>[4x]GAMGSRLYDRRSIFDAVAQSNCQELESLLPFLQRSKKRLTDSEFKDPETGKTCLLKAMLNLHNGQNDTIALLLDVARKTDSLKQFVNASYTDSYYKGQTALHIAIERRNMTLVTLLVENGADVQAAANGDFFKKTKGRPGFYFGELPLSLAACTNQLAIVKFLLQNSWQPADISARDSVGNTVLHALVEVADNTVDNTKFVTSMYNEIL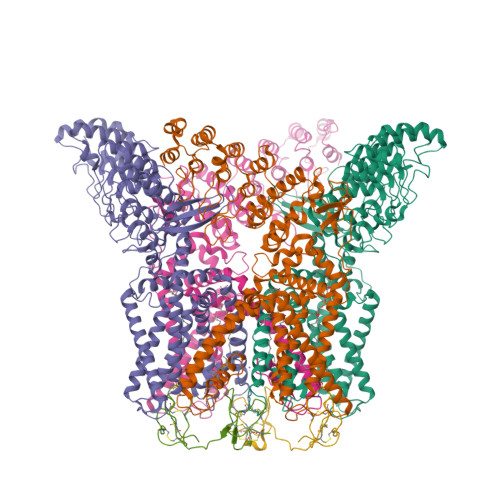ILGAKLHPTLKLEEITNRKGLTPLALAASSGKIGVLAYILQREIHEPECRHLSRKFTEWAYGPVHSSLYDLSCIDTCEKNSVLEVIAYSSSETPNRHDMLLVEPLNRLLQDKWDRFVKRIFYFNFFVYCLYMIIFTAAAYYRPVEGLPPYKLKNTVGDYFRVTGEILSVSGGVYFFFRGIQYFLQRRPSLKSLFVDSYSEILFFVQSLFMLVSVVLYFSQRKEYVASMVFSLAMGWTNMLYYTRGFQQMGIYAVMIEKMILRDLCRFMFVYLVFLFGFSTAVVTLIEDGKYNSLYSTCLELFKFTIGMGDLEFTENYDFKAVFIILLLAYVILTYILLLNMLIALMGETVNKIAQESKNIWKLQRAITILDTEKSFLKCMRKAFRSGKLLQVGFTPDGKDDYRWCFRVDEVNWTTWNTNVGIINEDPG;>[2x]MDCAKEGEVCSWGKKCCDLDNFYCPMEFIPHCKKYKPYVPVTTNCAKEGEVCGWGSKCCHGLDCPLAFIPYCEKYR> KDQPRPAFSAIRRNPPMGGNVVIFDTVITNQEEPYQNHSGRFVCTVPGYYYFTFQVLSQWEICLSIVSSSRGQVRRSLGFCDTTNKGLFQVVSGGMVLQLQQGDQVWVEKDPKKGHIYQGS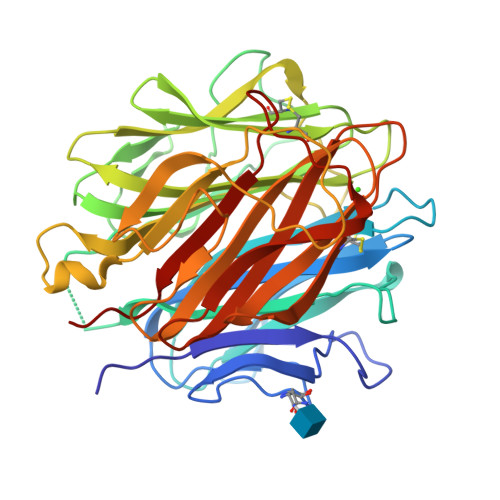EADSVFSGFLIFPSAGSGKQKFQSVFTVTRQTHQPPAPNSLIRFNAVLTNPQGDYDTSTGKFTCKVPGLYYFVYHASHTANLCVLLYRSGVKVVTFCGHTSKTNQVNSGGVLLRLQVGEEVWLAVNDYYDMVGIQGSDSVFSGFLLFPDGSAKATQKIAFSATRTINVPLRRDQTIRFDHVITNMNNNYEPRSGKFTCKVPGLYYFTYHASSRGNLCVNLMRGRERAQKVVTFCDYAYNTFQVTTGGMVLKLEQGENVFLQATDKNSLLGMEGANSIFSGFLLFPDMEA Ndc80c, a heterotetramer of Ndc80, Nuf2, Spc24, and Spc25, is a 600 Å long rod, largely two-chain coiled-coil, with an Ndc80/Nuf2 globular “head” at one end and an Spc24/Spc25 globular knob at the other. The Mps1 and Aurora B kinases regulate and monitor kinetochore attachment to spindle microtubules during cell division, ultimately ensuring accurate chromosome segregation. We show here, biochemically and structurally, that short peptide segments on both Mps1 and Ipl1 bind the site on the Ndc80/Nuf2 head of Ndc80c that we have shown previously to bind an Ipl1-phosphoregulated peptide segment near the C-terminus of Dam147. The Ndc80c head is thus a communication hub for ensuring a robust linkage between centromere and spindle and for integrating the SAC with tension sensing and error correction.

We applied the strategy we used to determine the Dam1-Ndc80c interaction, by generating chimeras with the C-terminus of the Mps1 peptide joined to the N-terminus of Nuf2 as a continuous polypeptide chain. The Mps1: Ndc80cdwarf chimera crystallized in space group C2221 (a = 72.5 Å, b = 168.5 Å, c = 229.6 Å). We recorded diffraction data to a minimum Bragg spacing of 2.9 Å and determined the structure as described in Methods. The N-terminal seven residues of the motif (RRSKRFL) form a short helix, which has a set of contacts with conserved glutamate residues in αH of Ndc80 and with conserved features of Nuf2. In the crystal structure, the guanidinium groups of R152 and R154 both bridge to the carboxylate of Ndc80 E166, and the side-chain NH3+ of K153 projects to the carboxylate of Ndc80 E162. The conserved phenylalanine, Mps1 F156, inserts into a hydrophobic pocket lined by Ndc80 L169, L170 and F172, and Nuf2 M154, with a further contribution from Mps1 L157. The C-terminal six residues of the Mps1 motif (LGPAKR) extend across Nuf2 αG, with contacts from residues 128 and 130–132 (conserved in point-centromere yeast). N128, conserved not only in yeasts but also in metazoans, anchors the end of the motif with hydrogen bonds between its side-chain amide and the main-chain amide and carbonyl of K169 (the penultimate residue in the motif), thus mimicking the hydrogen bonds in an antiparallel β-sheet. This interaction positions the invariant arginine of the motif to salt bridge with Ndc80 D295, likewise conserved in both metazoans and yeast. Residues F8 and P9 together bury the hydrogen-bonding interactions of N128 with the main chain of the penultimate residue in the Mps1 and Dam1 binding motifs and probably contribute both to the strength of those interactions and to correct positioning of the invariant arginine to salt bridge with Ndc80 D295.

> SNARDPRPLRDKNFQSAIQEEIYDYLKKNKFDIETNHPISIKFLKQPTQKGFIIIFKWLYLRLDPGYGFTKSIENEIYQILKNLRYPFLESINKSQISAVGGSNWHKFLGMLHWMVRTNIKLDMCLNKVDRSLINQNTQEITILSQPLKTLDEQDQRQERYELMVEKLLIDYFTESYKSFLKLEDNYEPSMQELKLGFEKFVHIINTDVTSTELKLEELKVDLNRKRYKLHQQVIHVIDITSKFKINIQSSLENSENELGNVIEELRNLEFETEHNVTN;> MRQNMKEDITAKYAERRSKRFLISNRTTKLGPAKRASRNQDVFPILDLQELVICLQSCDFALATQENISRPTSDYMVTLYKQIIENFMGISVESLLNSSNQETGDGHLQEENENIYLDTLNVLVLNKICFKFFENIGVQDFNMTDLYKPEAQRTQRLLSAVVNYARFREERMFDCNSFILQMESLLGQINKLNDEIKQLQKDFEVEVKEIEIEYSLLSGHINKYMNEMLEYMQ;> MSQKDNLLDNPVEFLKEVRESFDIQQDVDAMKRIRHDLDVIKEESEARLKLYRSLGVILDLENDQVLINRKNDGNIDILPLDNNLSDFYKTKYIWERLGK;> MASIDAFSDLERRMDGFQKDVAQVLARQQNHVALYERLLQLRVLPGASDVHDVRFVFGDDSRCWIEVAMHGDHVIGNSHPALDPKSRATLEHVLTVQGDLAAFLVVARDMLLASL> STNMLEALQQRLEK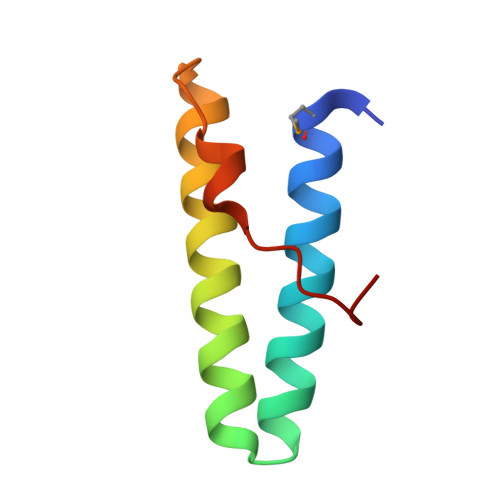YQSVEAAAKAENNSGKARRFGRIVKQYEDAIKLYKAGKPVPYDELPVPPGFG>[4x]SVDLIGINVAGAEFTGGKLPGKHGTHYFFPPEGYFEYWSEQGIHTVRFPLKWERLQPSLNAELDDVYASLVDDMLDQAKENDIKVILDVHNYARYRKKVIGTEDVPVSAYQDLMERIAKRWQGHDALFAYDIMNEPYGSADKLWPAAAQAGIDGVRKYDKKRPLLIEGASWSSAARWPRYADELLKLKDPADNMVFSAHVFIDEDASGSYKKGPGKDF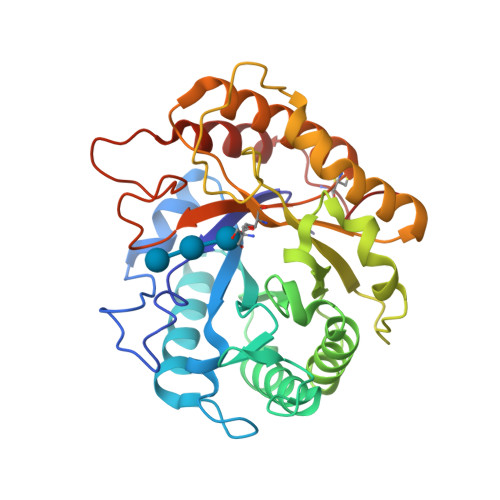EPMIGVKRVEPFVNWLKEHGKKGHIGEFGIPNDDERWLDAMDKLLAYLNENCIPINYWAAGPSWGNYKLSIEPKDGEKRPQVALLKKYAAKDNCSDFGPAKA> ADDALAALGAQLFVDPALSRNATQSCATCHDPARAFTDPREGKAG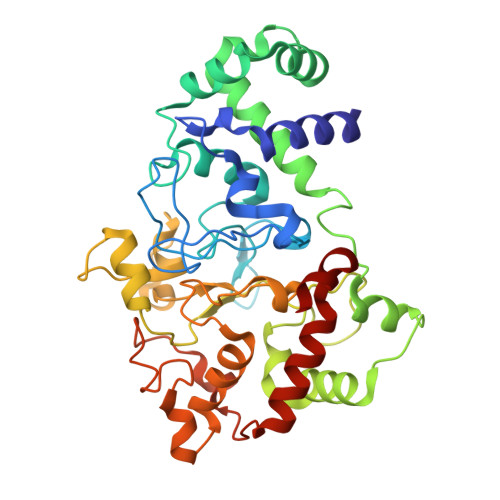LAVSVGDDGQSHGDRNAPTLGYAALVPAFHRDANGKYKGGQFWDGRADDLKQQAGQPMLNPVEMAMPDRAAVAARLRDDPAYRTGFEALFGKGVLDDPERAFDAAAEALAAYQATGEFSPFDSKYDRVMRGEEKFTPLEEFGYTVFITWNCRLCHMQRKQGVAERETFTNFEYHNIGLPVNETAREASGLGADHVDHGLLARPGIEDPAQSGRFKVPSLRNVAVTGPYMHNGVFTDLRTAILFYNKYTSRRPEAKINPETGAPWGEPEVARNLSLAELQSGLMLDDGRVDALVAFLETLTDRRYEPLLEE>GMTTRKPFIICDFDGTITMNDNIINIMKTFAPPEWMALKDGVLSKTLSIKEGVGRMFGLLPSSLKEEITSFVLEDAKIREGFREFVAFINEHEIPFYVISGGMDFFVYPLLEGIVEKDRIYCNHASFDNDYIHIDWPHSCKGTCSNQCGCCKPSVI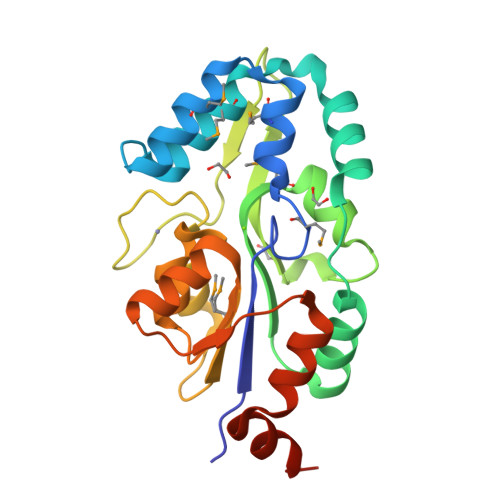HELSEPNQYIIMIGDSVTDVEAAKLSDLCFARDYLLNECREQNLNHLPYQDFYEIRKEIENVKEVQEWLQNKNAGESSLK[2x]>MSQVTDMRSNSQGLSLTDSVYERLLSERIIFLGSEVNDEIANRLCAQILLLAAEDASKDISLYINSPGGSISAGMAIYDTMVLAPCDIATYAMGMAASMGEFLLAAGTKGKRYALPHARILMHQPLGGVTGSAADIAIQAEQFAVIKKEMFRLNAEFTGQPIERIEADSDRDRWFTAAEALEYGFVDH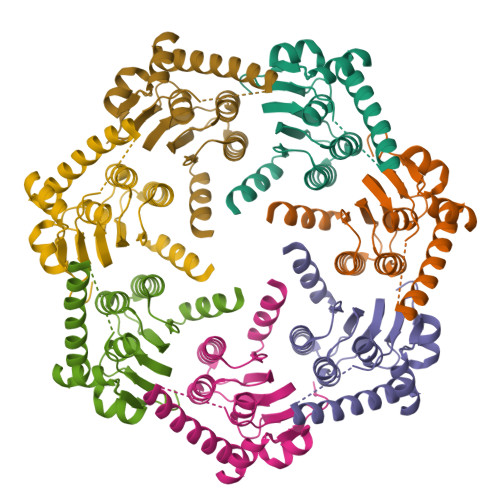IITRAHVNGEAQLEHHHHHH[7x]> MGFHMKGADGISPPLTYRSWHIEGGQ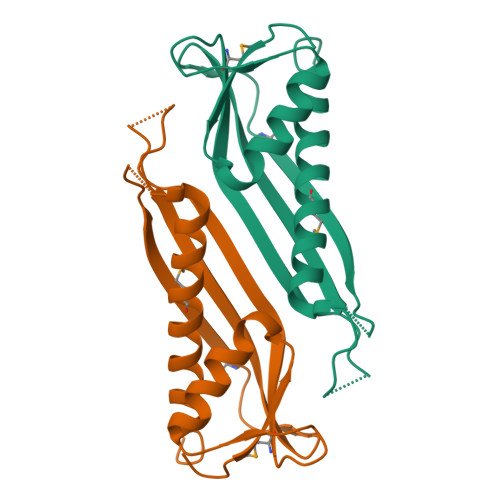ALQFPLETALYQASGRVDDAAGAQMTLRIDSVSQNKETYTVTRAAVINEYLLILTVEAQVLKRGEPVGKPMTVSVRRVLAYADNEILGKQEEEAALWAEMRQDAAEQIVRRLTFLKAELEHHHHHH>GPGSMMVLYSGTTCPFSQRCRLVLFEKGMDFEIRDVDLFNKPEDISVMNPYGQVPILVERDLILYESNIINEYIDERFPHPQLMPADPVQRARARLFLLNFEKELFVHVSTLENEKGKAAEKNHEKARLAIRDRLTQLAPIFVKN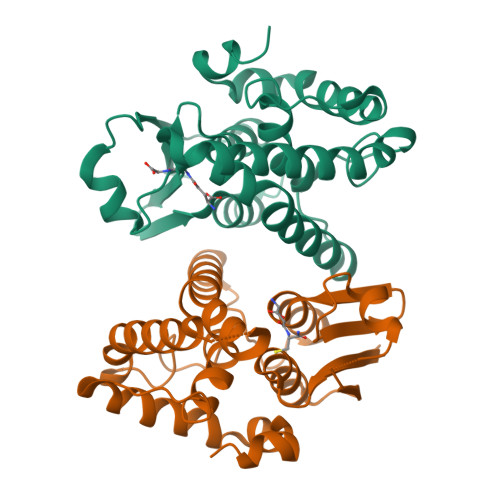KYMLGEEFSMLDVAIAPLLWRLDHYGIELSKNAAPLMKYAERIFSRPAYIEALTPSEKVMRR[2x]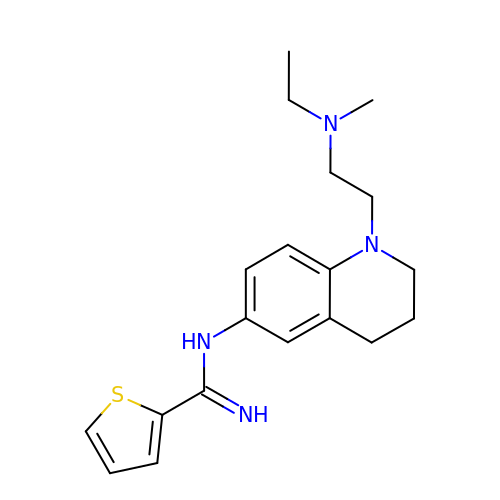N-(1-{2-[ethyl(methyl)amino]ethyl}-1,2,3,4-tetrahydroquinolin-6-yl)thiophene-2-carboximidamide | C19 H26 N4 S | GDMWZTBOBNMXTL-UHFFFAOYSA-N> LKKQYIFQLSSLNPQERIDYCHLIEKLGGLVIEKQCFDPTCTHIVV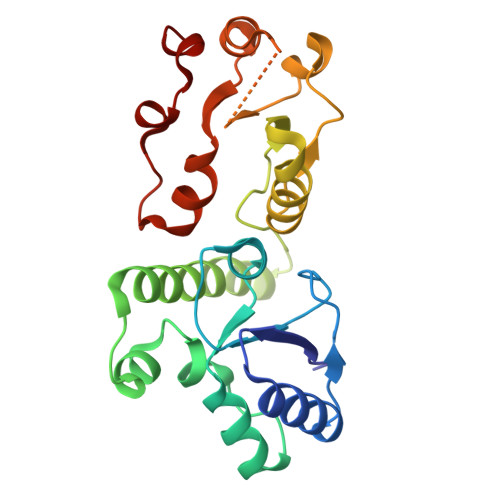GHPLRNEKYLASVAAGKWVLHRSYLEACRTAGHFVQEEDYEWGSSSILDVLTGINVQQRRLALAAMRWRKKIQQRQESGIVEGAFSGWKVILHVDQSREAGFKRLLQSGGAKVLPGHSVPLFKEATHLFSDLNKLKPDDSGVNIAEAAAQNVYCLRTEYIADYLMQESPPHVENYCLPEAISFI> MDMMMDKQEIKREY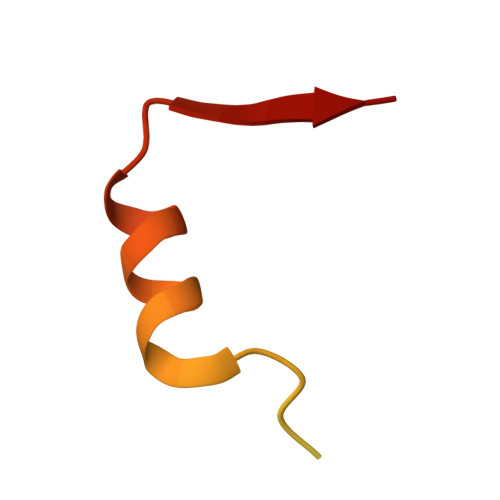IEQEGHFETKSRRRELHIEILSEQTKSDIRNSKLVVMN> GHMHNTELLPIELDTLVGKGRFAEVYKAKLKQNTSEQFETVAVKIFPYEEYASWKTEKDIFSDINLKHENILQFLTAEERKTELGKQYWLITAFHAKGNLQEYLTRHVISWEDLRKLGSSLARGIAHLHSDHTPCGRPKMPIVHRDLKSSNILVKNDLT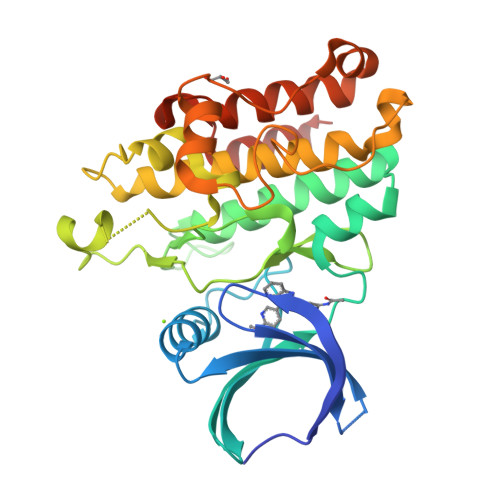CCLCDFGLSLRLDPTLSVDDLANSGQVGTARYMAPEVLASAMNLENVESFKQTDVYSMALVLWEMTSRCNAVGEVKDYEPPFGSKVREHPCVASMADNVLADAGRPEIPSFWLNHQGIQMVCETLTECWDHDPEARLTAQCVAERFSELEHLDRLSG> AGVMTGAKFTQIQFGMTRQQVLDIAGAENCETGGSFGDSIHCRGHAAGDYY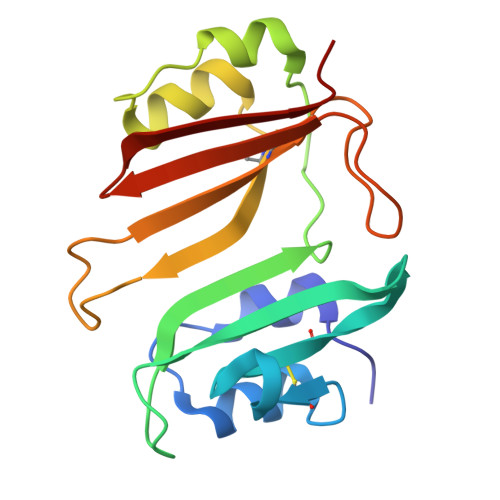AYATFGFTSAAADAKVDSKSQEKLLAPSAPTLTLAKFNQVTVGMTRAQVLATVGQGSCTTWSEYYPAYPSTAGVTLSLSCFDVDGYSSTGAYRGSAHLWFTDGVLQGKRQWDLV The activity of σ factors is often regulated by their association with an anti-σ factor. Mtb RslA is a ZAS protein with a cytosolic domain (ASD) that interacts with the ECF σ factor σL and a membrane-spanning C-terminal domain. With in vitro transcription assays, the anti-σ factor of σL, RslA, was shown to inhibit σL-dependent transcription of the σB gene in a dose-dependent manner. RslA responds to oxidative stimuli with the release of the Zn2+ cofactor, followed by the formation of a disulfide link between proximal cysteines of the HXXXCXXC motif.

Crystals were readily obtained from an expression construct that had σ4L and RslA. There are 10 molecules of the σ4L/RslA complex in the asymmetric unit. In this arrangement, five heterotetramers of the σ4L/RslA complex pack with a 5-fold symmetry to form a ring-like structure, with the zinc binding region of RslA facing the center of the ring. The 1:1 stoichiometry for the σ4L/RslA complex seen in the crystal structure is consistent with biochemical data. About 23 residues in the N-terminus and 22 residues in the C-terminus were disordered in the crystal structure of RslA. σ4L forms a tight complex with RslA involving a buried surface area of ca 1332 Å2. The Zn2+ cofactor in RslA is coordinated by His25, His50, Cys54, and Cys57. Thus, all the conserved residues in the HXXXCXXC motif are involved in Zn2+ binding. The crystal structure shows that the orientation of domains in the σ4L/RslA complex is different from that in Rsp ChrR, the only other structurally characterized ZAS–σ factor complex. Unlike Rsp ChrR, no structural rearrangements were seen in σ4L upon RslA binding. In summary, the crystal structure of the σ4L/RslA complex reveals that RslA inactivates σL by sterically occluding both the promoter and the RNAP binding regions on σ4L.

>[10x]MGSSHHHHHHSQDPEQSTPDEVNAALDRLLIADALAQLSAEHRAVIQRSYYRGWSTAQIATDLGIAEGTVKSRLHYAVRALRLTLQELGVTR;>MTMPLRGLGPPDDTGVREVSTGDDHHYAMWDAAYVLGALSAADRREFEAHLAGCPECRGAVTELCGVPALLSQLDRDEVAAISESAPTVVASGLSPELLPSLLAAVHR[10x]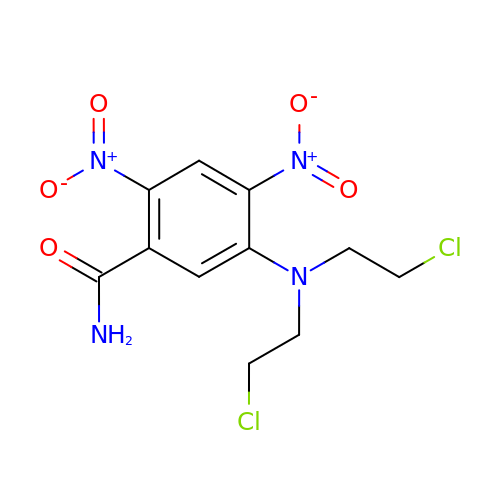5-[BIS-2(CHLORO-ETHYL)-AMINO]-2,4-DINTRO-BENZAMIDE | C11 H12 Cl2 N4 O5 | DQMALWRRERBILB-UHFFFAOYSA-N2-chloroethane-1-sulfonic 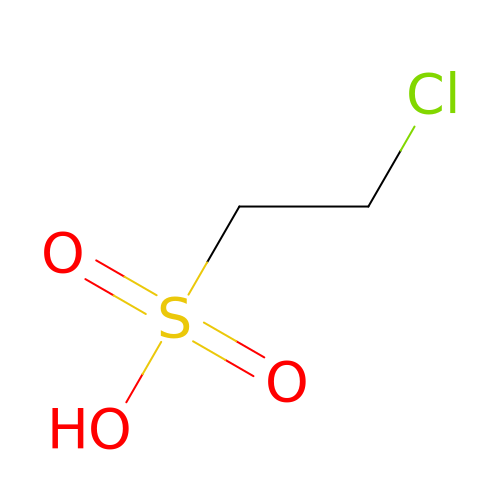acid | C2 H5 Cl O3 S | FXKMTSIKHBYZSZ-UHFFFAOYSA-N>[2x]MDIWYGTAAVPKDLDNSAVTIGVFDGVHRGHQKLINATVEKAREVGAKAIMVTFDPHPVSVFLPRAAPLGITTLAERFALAESF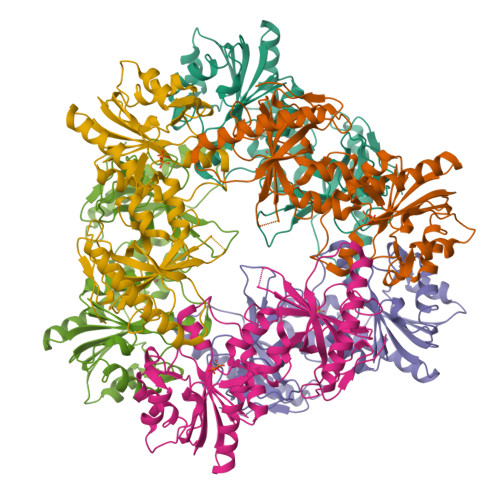GIDGVLVIDFTRELSGTSPEKYVEFLLEDTLHASHVVVGANFTFGENAAGTADSLRQICQSRLTVDVIDLLDDEGVRISSTTVREFLSEGDVARANWALGRHFYVTGPVVRGAGRGGKELGFPTANQYFHDTVALPADGVYAGWLTILPTEAPVSGNMEPEVAYAAAISVGTNPTFGDEQRSVESFVLDRDADLYGHDVKVEFVDHVRAMEKFDSVEQLLEVMAKDVQKTRTLLAQDVQAHKMAPETYFLQAES> MSESLLYGYFLD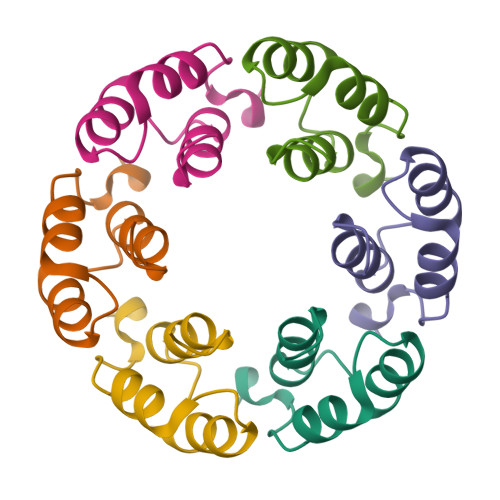SWLDGTASEELLRVAVNAGDLTQEEADKIMSYPWGAWND>[2x]AGPWADIMQGPSESFVDFANRL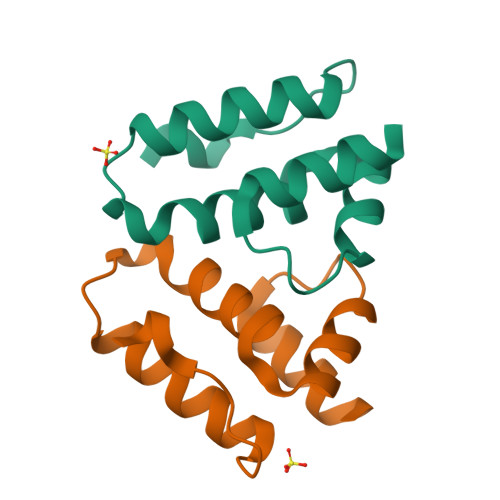IKAVEGSDLPPSARAPVIIDCFRQKSQPDIQQLIRTAPSTLTTPGEIIKYVLDRQ>[4x]MGHHHHHHSHMDEQSVESIAE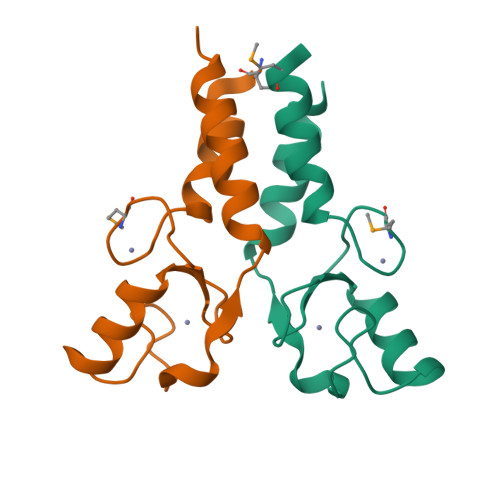VFRCFICMEKLRDARLCPHCSKLCCFSCIRRWLTEQRAQCPHCRAPLQLRELVNCRWAEEVTQQLDTLQLCSLTKHEEN>A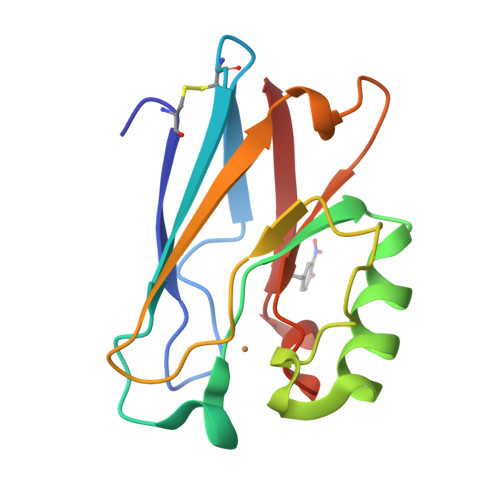ECSVDIQGNDQMQFNTNAITVDKSCKQFTVNLSHPGNLPKNVMGHNFVLSTAADMQGVVTDGMASGLDKDFLKPDDSRVIAQTKLIGSGEKDSVTFDVSKLKEGEQFMFFCTFPGHSALMYGHLTLK[2x]> AGCSDVSTELKTPVYKTKLTAEEIRNSAFKPEFPKQYASYERNDETTVMTEYKGSVPFNKNDNVNPLPEGYRHAQPYLKNLWLGYPFMYEYREARGHTYAIQDFLHIDRINRYAEKGGLPATCWNCKTPKMMEWVKESGDGFWAKDVNEFRDKIDMK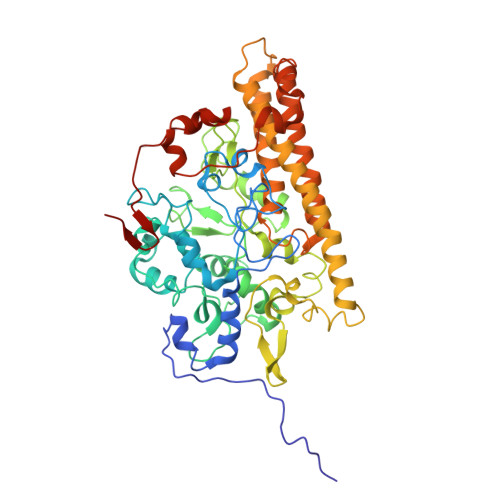DHTIGCATCHDPQTMELRITSVPLTDYLVSQGKDPKKLPRNEMRALVCGQCHVEYYFNGPTMGVNKKPVFPWAEGFDPADMYRYYDKHGDLQVKGFEGKFADWTHPASKTPMIKAQHPEYETWINGTHGAAGVTCADCHMSYTRSDDKKKISSHWWTSPMKDPEMRACRQCHSDKTPDYLKSRVLFTQKRTFDLLLAAQEVSVKAHEAVRLANEYQGAKAAGYDDLMIQAREMVRKGQFFWDYVSAENSVGFHNPAKALDTLAQSQQFSQKAIDLAMEATQYGIGKDLSGDIKTIVPPILKMNRKLQQDPEFMKTHKWFQYLPVLPKADQVWDGQKRLVSAKQ Secretory (S) Immunoglobin (Ig) A is the predominant, mammalian mucosal antibody; it is a polymeric antibody assembled in plasma cells that link two IgA monomers and a single copy of the joining chain (JC) to form dimeric (d) IgA (and to a lesser extent, higher order polymers). The pIgR uses five Ig-like domains (D1-D5) and a cytoplasmic tail to bind and transcytose JC-containing antibodies to the apical surface of epithelial cells; there, the pIgR ectodomain, called secretory component (SC), is proteolytically cleaved, releasing the SC-dIgA complex into the mucosa where it is called SIgA (Stadtmueller et al., 2016a). The IgA CH3 contains a C-terminal extension called the tailpiece (Tp), which along with the JC, is required for IgA dimerization and subsequent pIgR binding. Our work describes the structures of mouse SIgA and its precursor, dIgA, which lacks the SC.

We determined the CryoEM structure of mouse SIgA to a final average resolution of 3.3 Å. The refined structure revealed a pseudosymmetric assembly of two IgA monomers conjoined at the center by the JC and bound by SC. The FcAB and FcCD are bent and tilted with respect to each other, resulting in distinct concave and convex surfaces on the complex. To describe the conformation, we defined the angle between the centroid axes of FcAB and FcCD (97 degrees) as ‘bend’, and the angle between the two non-intersecting centroid planes of FcAB and FcCD (30 degrees) as ‘tilt’. SC asymmetrically contacts the same face of both FcAB and FcCD along what we define as the ‘front face’ of the molecule. The interface is dominated by the four heavy chain Tps (TpA, TpB, TpC, TpD) and the first half of the JC sequence, or, ‘core’ (JCcore), which together fold into a single β-sandwich-like domain at the center of the complex. The interface is further stabilized by the second half of the JC sequence, which folds into two beta-hairpin ‘wings’ (JCW1 and JCW2), each extending outward from the center of the complex and binding one CH3 from each IgA monomer. In contrast to unliganded SC, the SIgA structure reveals SC domains bound to dIgA in an elongated, open conformation contacting both antibodies and the JC asymmetrically on the front face of the complex. D1 contacts FcAB, FcCD and the JC, D2 protrudes away from other SC domains and the front face of the molecule, and D3 is clamped to D1, positioning D4 and D5 to contact FcCD and JCW1. The interface is dominated by residues in D5 CDR1, including Cys470, which disulfide bonds to CH2C Cys306, covalently linking SC to the antibody, as well as D5 CDR1 Lys471 and Tyr473, which form hydrogen bonding and hydrophobic interactions with CH2C.

>[4x]WGQGTLVTVSAESARNPTIYPLTLPPALSSDPVIIGCLIHDYFPSGTMNVTWGKSGKDITTVNFPPALASGGRYTMSSQLTLPAVECPEGESVKCSVQHDSNPVQELDVNCSGPTPPPPITIPSCQPSLSLQRPALEDLLLGSDASITCTLNGLRNPEGAVFTWEPSTGKDAVQKKAVQNSCGCYSVSSVLPGCAERWNSGASFKCTVTHPESGTLTGTIAKVTVNTFPPQVHLLPPPSEELALNELLSLTCLVRAFNPKEVLVRWLHGNEELSPESYLVFEPLKEPGEGATTYLVTSVLRVSAETWKQGDQYSCMVGHEALPMNFTQKTIDRLSGKPTNVSVSVIMSEGDGICY;> KSPIFGPQEVSSIEGDSVSITCYYPDTSVNRHTRKYWCRQGASGMCTTLISSNGYLSKEYSGRANLINFPENNTFVINIEQLTQDDTGSYKCGLGTSNRGLSFDVSLEVSQVPELPSDTHVYTKDIGRNVTIECPFKRENAPSKKSLCKKTNQSCELVIDSTEKVNPSYIGRAKLFMKGTDLTVFYVNISHLTHNDAGLYICQAGEGPSADKKNVDLQVLAPEPELLYKDLRSSVTFECDLGREVANEAKYLCRMNKETCDVIINTLGKRDPDFEGRILITPKDDNGRFSVLITGLRKEDAGHYQCGAHSSGLPQEGWPIQTWQLFVNEESTIPNRRSVVKGVTGGSVAIACPYNPKESSSLKYWCRWEGDGNGHCPVLVGTQAQVQEEYEGRLALFDQPGNGTYTVILNQLTTEDAGFYWCLTNGDSRWRTTIELQVAEATREPNLEVTPQNATAVLGETFTVSCHYPCKFYSQEKYWCKWSNKGCHILPSHDEGARQSSVSCDQSSQLVSMTLNPVSKEDEGWYWCGVKQGQTYGETTAIYIAVEER;> DDEATILADNKCMCTRVTSRIIPSTEDPNEDIVERNIRIVVPLNNRENISDPTSPLRRNFVYHLSDVCKKCDPVEVELEDQVVTATQSNICNEDDGVPETCYMYDRNKCYTTMVPLRYHGETKMVQAALTPDSCYPD>KSQYLEKINEVIRRAWAVPTHGHELGYSLCNSLRQSGGLDLLMKNCVKPDLQFSSAQLLEQCLTTENRKHVVDNGLDKVVNVACVCTKNSNMEHSRVGTGILEHLFKHSEGTCSDVIRLGGLDAVLFECRTSDLETLRHC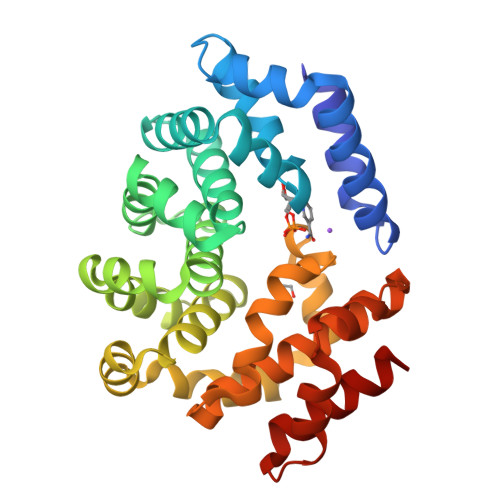ASALANLSLYGGAENQEEMILRKVPMWLFPLAFHNDDNIKYYACLAIAVLVANKEIEAEVLKSGCLDLVEPFVTSHDPSAFARSNLAHAHGQSKHWLKRLVPVLSSNREEARNLAAFHFCMEAGIKREQGNTDIFREINAIEALKNVASCPNAIASKFAAQALRLIGET[2x]>[30x]MTDFYTIKDAQADLAIAPLNLTVLLAPYSTTPATTLESPTDGSLAIPPGYKSVGHFEKQAGLTLGNEFDSKDIEAYGEPEPIRTIINKRTTTFDFAMYQNQRNVLELIWTQDFSNIQPSEFGGIVLEAPKVPKNIYYRAILVGMDDRNDRPIWLYWLMPKVKLDKLDNQTLNDDNVIEYKPTLKAFRDDVVGYSVAQGFAGPGWRDLVATAGFGEALTALTITPGSPTVTVA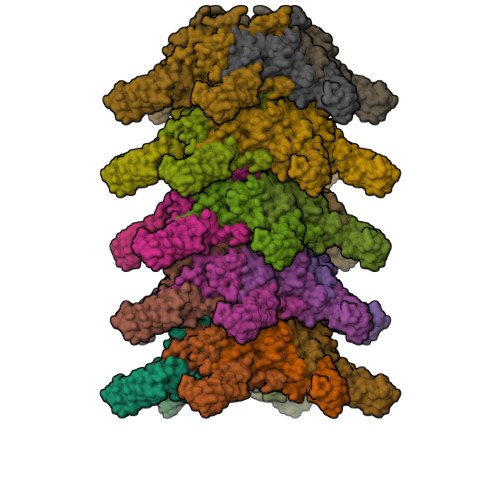TGASHTAQLLVEGDNGINYTPDVVFTSSAPDKASVSAAGLVTGVAAGSATITATKGALTATATVTVTA> MGITAPTPLTSEHNLADFCCSDHGMNEWLKKKALKNHSSGLSRVYVICIANTRQVIGYYCLSTGSIQRNLAPGAMR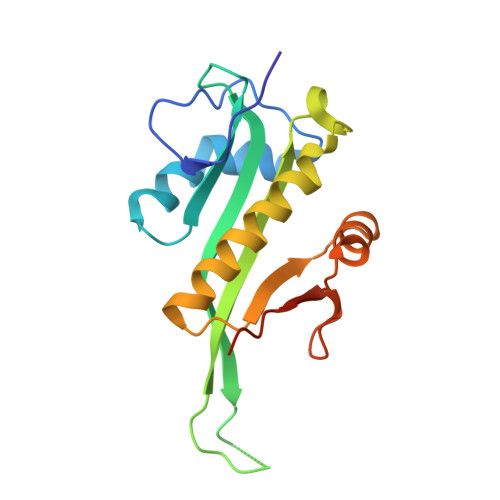RNAPESLPVVVLGRLAIDQAWAGKGLGVALLKDAVYRTMSIAQQVGVRALIVHALDDSVRNFYLKYAFVPSPFQSLTLLYPITLELEHHHHHH> TAPSQVLKIRRPDDWHLHLRDGDMLKTVVPYTSEIYGRAIVMPNLAPPVTTVEAAVAYRQRILDAVPAGHDFTPLMTCYLTDSLDPNELERGFNEGVFTAAKLYPANASTNSSHGVTSVDAIMPVLERMEKIGMPLLVHGEVTHADIDIFDREARFIESVMEPLRQRLTALKVVFEHITTKDAADYVRDGNERLAATITPQHLMFNRNHMLVGGVRPHLYCLPILKRNIHQQALRELVASGFNRVFLGTDSAPHARHRKESSCGCAGCFNAPTALGSYATVFEEMNALQHFEAFCSVNGPQFYGLPVN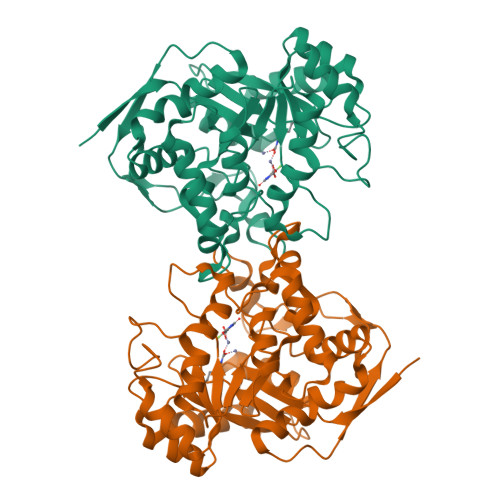DTFIELVREEQQVAESIALTDDTLVPFLAGETVRWSVKQ>AGFQLNEFSSSGLGRAYSGEGAIADDAGNVSRNPALITMFDRPTFSAGAVYIDPDVNISGTSPSGRSLKADNIAPTAWVPNMHFVAPINDQFGWGASITANDLATEFNDTYAGGSVGGTTDLETMNLNLSGAYRLNNAWSFGLGFNAVYARAKIERFAGDLGQLVAGQIMQSPAGQTQQGQALAATANGIDSNTKTAHLNGNQWGFGWNAGILYELDKNNRYALTYRSEVKIDFKGNYSSDLNRAFNNYGLPIPTATGGATQSGYLTLNLPEMWEVSGYNRVDPQWAIHYSLAYTSWSQFQQLKATSTSGDTL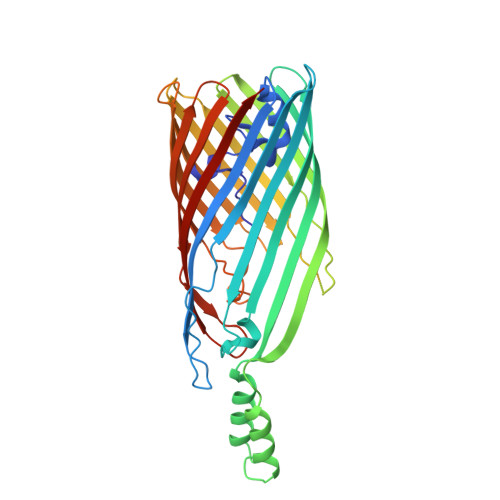FQKHEGFKDAYRIALGTTYYYDDNWTFRTGIAFDDSPVPAQNRSISIPDQDRFWLSAGTTYAFNKDASVDVGVSYMHGQSVKINEGPYQFESEGKAWLFGTNFNYAFHHHHHH[2x]> GAPHEERVGDMRIVNITFSDINSIKNFQPFSQYFDFTLTGPRYNGNIAQFAMIWKIKNPPHNLLGVFFDNNTRDDE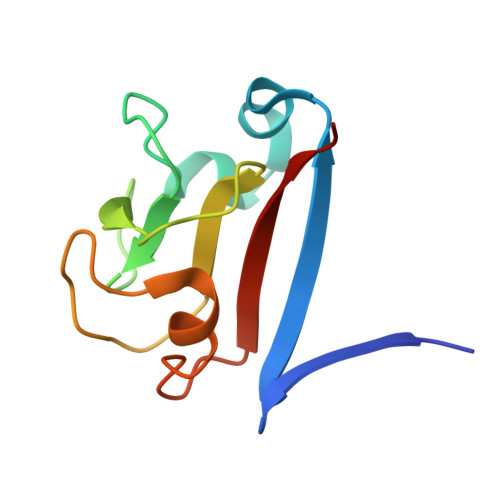DDKYTLEELKQMGNGAKNMYIFWQYEQK>SNAMNKTLIINAHPKVDDTSSVSIKVFKHFLESYKELISNNETIEQINLYDDVVPMIDKTVLSAWEKQGNGQELTREEQKVTERMSEILQQFKSANTYVIVLPLHNFNIPSKLKDYMDNIMIARETFKYTETGSVGLLKDGRRMLVIQASGGIYTNDDWYTDVEYSHKYLKAMFNFLGIEDYQIVRAQGTAVLDPTEVLQNAYKEVEEAASRLANK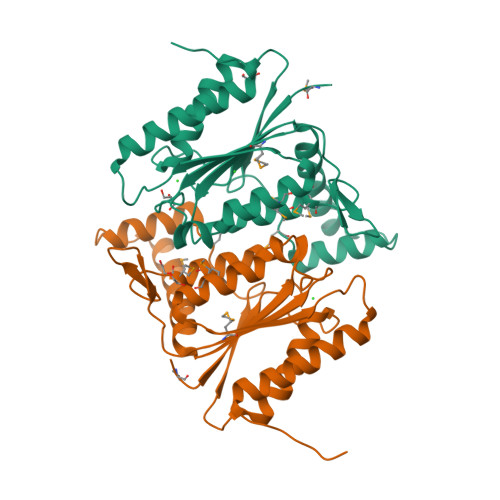YIFSLEE[4x]>NDLVFSSWGGTTQDAQ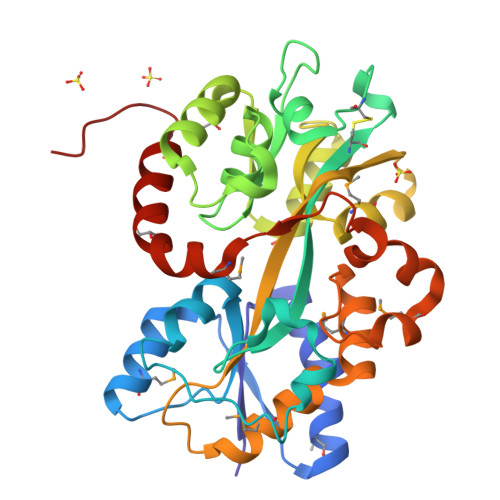KAAWAEKFMVETGINVLQDGPTDYGKLKAMVEANGVTWDVVDVEGDYAAQAGPKGLLEKLDFSVIDKTKLDPRFVTDYSVGSFYYSFVIGCNVDSVSACPKSWADLFDTAKFPGKRTFYKWSAPGVIEAALLADGVTADKLYPLDLDRAFKKLDTIKSDIIWWSGGAQSQQLIASAEAPFGSVWNGRMTALEQSGVKVETSWAQNITAADSLVVPKGTKNKDAAMKFIALATSAQAQADMATATGYAPVNIESAKLMDPKIAKSLPDQQTESQVNADMNYWAQHRDEIGERWYAWQAKHHHHHH[2x]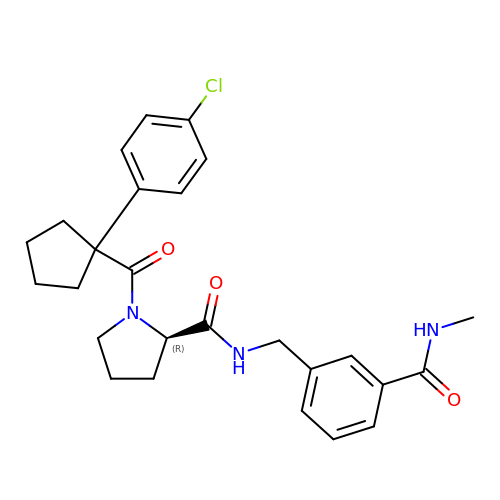1-[1-(4-chlorophenyl)cyclopentane-1-carbonyl]-N-{[3-(methylcarbamoyl)phenyl]methyl}-D-prolinamide | C26 H30 Cl N3 O3 | FKSCOWJURPRAGR-JOCHJYFZSA-N>MHYQPKQDLLNDRIILVTGASDGIGREAAMTYARYGATVILLGRNEEKLRQVASHINEETGRQPQWFILDLLTCTSENCQQLAQRIAVNYPRLDGVLHNAGLLGDVCPMSEQNPQVWQDVMQVNVNATFMLTQALLP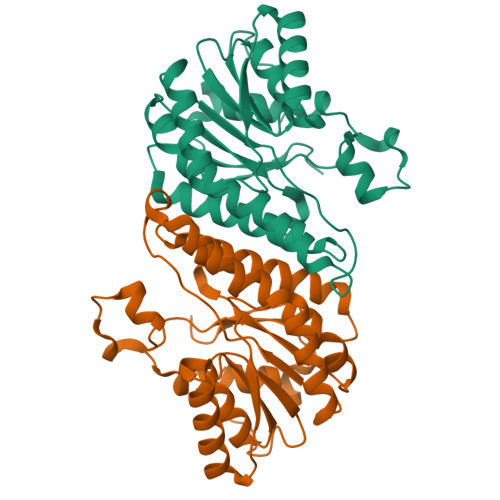LLLKSDAGSLVFTSSSVGRQGRANWGAYAASKFATEGMMQVLADEYQQRLRVNCINPGGTRTAMRASAFPTEDPQKLKTPADIMPLYLWLMGDDSRRKTGMTFDAQPGRKPGISQ[2x]>MHHHHHHTSKIEQPRWASKDSAAGAASTPDEKIVLEFMDALTSNDAAK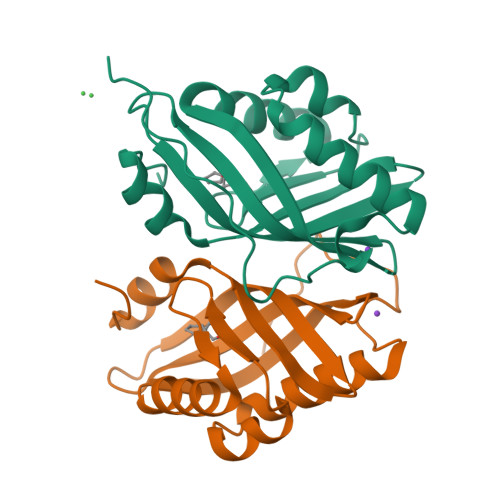LIEYFAEDTMYQNMPLPPAYGRDAVEQTLAGLFTVMSYDAVETFHIGSSNGLVYTERVDVLRALPTGKSYNVSVLGVFQLTEGKITGWRDYFDLREFEEAVDLPLRG[2x]>[2x]AQKSVKISDDISITQLSDKVYTYVSLAEIEGWGMVPSNGMIVINNHQAA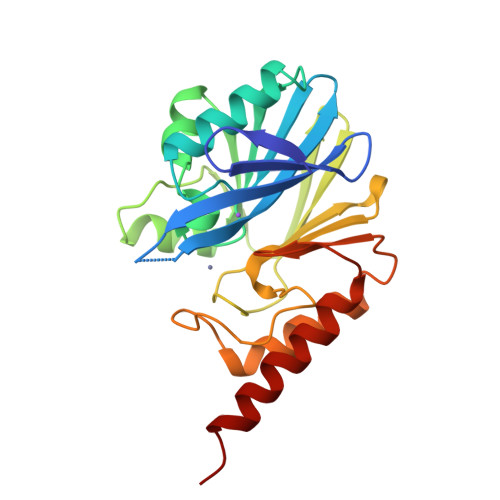LLDTPINDAQTETLVNWVADSLHAKVTTFIPNHWHGDCIGGLGYLQKKGVQSYANQMTIDLAKEKGLPVPEHGFTDSLTVSLDGMPLQCYYLGGGHATDNIVVWLPTENILFGGSMLKDNQATSIGNISDADVTAWPKTLDKVKAKFPSARYVVPGHGDYGGTELIEHTKQIVNQYIESTSKP>MTEYEGPKTKFHALMQEQIHNEFTAAQQYVAIAVYFDSEDLPQLAKHFYSQAVEERNHAMMLVQHLLDRDLRVEIPGVDTVRNQFDRPREALALALDQERTVTDQVGRLTAVARDEGDFLGEQFMQWFLQEQIEEVALMATLVRVADRAGANLFELENFVAREVDVAPAASGAPHAAG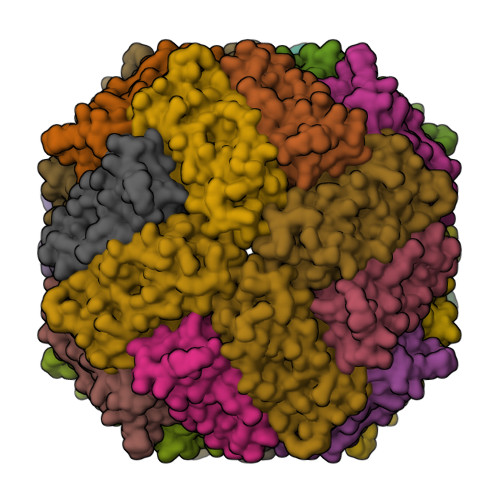GRL[24x]>MTALTESSTSKFVKINEKGFSDFNIHYNEAGNGETVIMLHGGGPGAGGWSNYYRNVGPFVDAGYRVILKDSPGFNKSDAVVMDEQRGLVNARAVKGLMDALDIDRAHLVGNSMGGATALNFALEYPDRIGKLILMGPGGLGPSMFAPMPMEGIKLLFKLYAEPSYETLKQMLQVFLYDQSLITEELLQGRWEAIQRQPE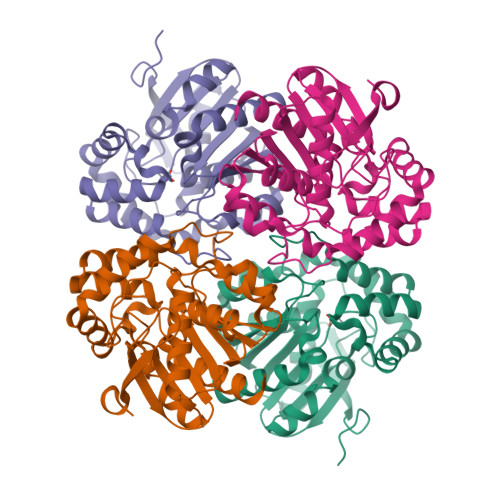HLKNFLISAQKAPLSTWDVTARLGEIKAKTFITWGRDDRFVPLDHGLKLLWNIDDARLHVFSKCGQWAQWEHADEFNRLVIDFLRHA[2x]> GAGEARLEEAVNRWVLKFYFHEALRAFRGSRYGDFRQIRDIMQALLVRPLGKEHTVSRLLRVMQCLSRIEEGENLDCSFDMEAELTPLESAINVLEMIKTEFTLTEAVVESSRKLVKEAAVIICIKNKEFEKASKILKKHMSKDPTTQKLRNDLLNIIREKNLAHPVIQNFSYETFQQKMLRF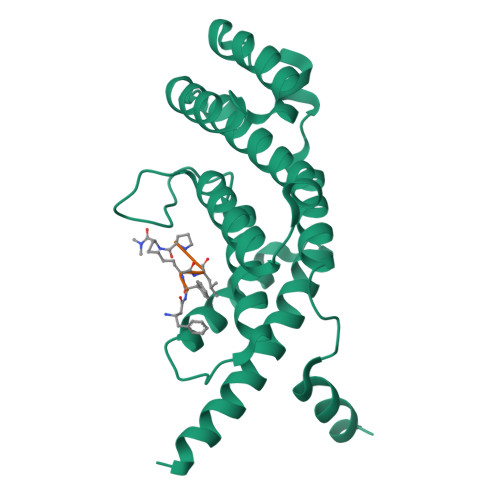LESHLDDAEPYLLTMAKKALK>[3x]SGSGENNRARPCDTCRSNACTVYCHADSA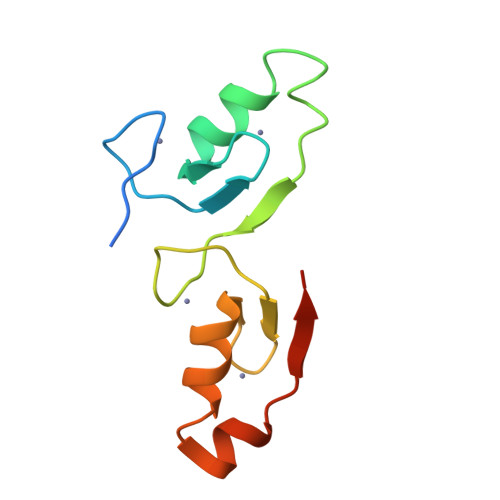YLCMSCDAQVHSANRVASRHKRVRVCESCERAPAAFLCEADDASLCTACDSEVHSANPLARRHQRVPILPISG> MIAAQLLAYYFTELKDDQVKKIDKYLYAMRLSDETLIDIMTRFRKEMKNGLSRDFNPTATVKMLPTFVRSIPDGSEKGDFIALDLGGSSFRILRVQVNHEKNQNVHMESEVYDTPENIVHGSGSQLFDHVAECLGDFMEKRKIKDKKLPVGFTFSFPCQQSKIDEAILITWTKRFKASGVEGADVVKLLNKAIKKRGDYDANIVAVVNDTVGTMMTCGYDDQH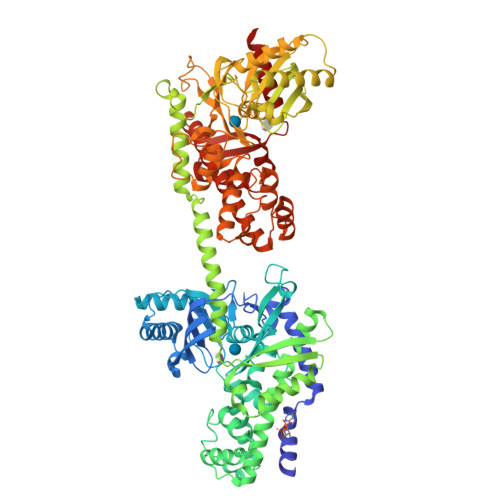CEVGLIIGTGTNACYMEELRHIDLVEGDEGRMCINTEWGAFGDDGSLEDIRTEFDRAIDAYSLNPGKQLFEKMVSGMYLGELVRLILVKMAKEGLLFEGRITPELLTRGKFNTSDVSAIEKNKEGLHNAKEILTRLGVEPSDDDCVSVQHVCTIVSFRSANLVAATLGAILNRLRDNKGTPRLRTTVGVDGSLYKTHPQYSRRFHKTLRRLVPDSDVRFLLSESGSGKGAAMVTAVAYRLAEQHRQIEETLAHFHLTKDMLLEVKKRMRAEMELGLRKQTHNNAVVKMLPSFVRRTPDGTENGDFLALDLGGTNFRVLLVKIRSGKKRTVEMHNKIYAIPIEIMQGTGEELFDHIVSCISDFLDYMGIKGPRMPLGFTFSFPCQQTSLDAGILITWTKGFKATDCVGHDVVTLLRDAIKRREEFDLDVVAVVNDTVGTMMTCAYEEPTCEVGLIVGTGSNACYMEEMKNVEMVEGDQGQMCINMEWGAFGDNGCLDDIRTHYDRLVDEYSLNAGKQRYEKMISGMYLGEIVRNILIDFTKKGFLFRGQISETLKTRGIFETKFLSQIESDRLALLQVRAILQQLGLNSTCDDSILVKTVCGVVSRRAAQLCGAGMAAVVDKIRENRGLDRLNVTVGVDGTLYKLHPHFSRIMHQTVKELSPKCNVSFLLSEDGSGKGAALITAVGVRLRTEASS> MEYKMRRERNNIAVRKSRDKAKMRNLETQHKVLELTAENERLQKKVEQL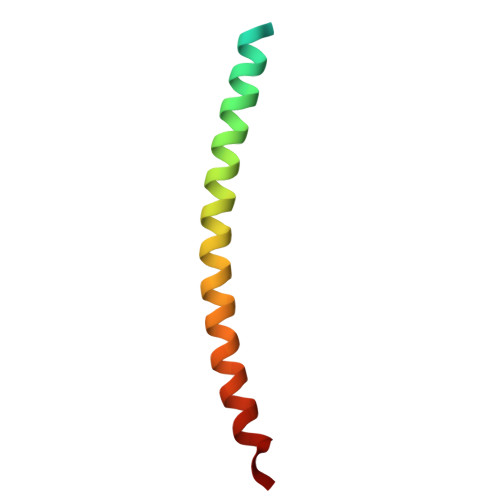SRELSTLRNLFKQL>GSKKIDDDLFEELEEQLLIADVGVETTR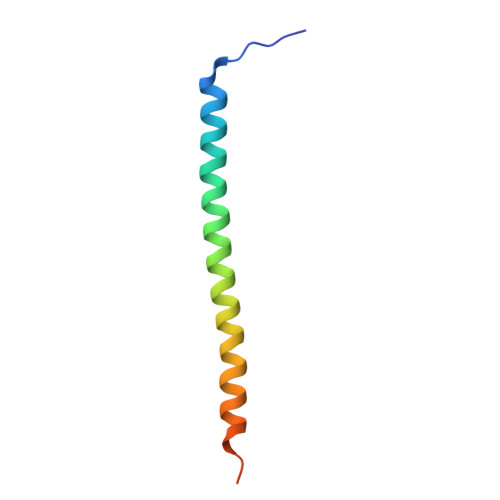KIITNLTEGASRKQLRDAEALYGLLKEEMGEILA[2x]>SRPHQWQTDEEGVRTGKCSFPVKYLGHVEVDESRGMHICEDAVKRLKAERKFFKGFFGKTGKKAVKAVLWVSADGLRVVDEKTKDLIVDQTIEKVSFCAPDRNFDRAFSYICRDGTTRRWICHCFMAVKDTGERLSH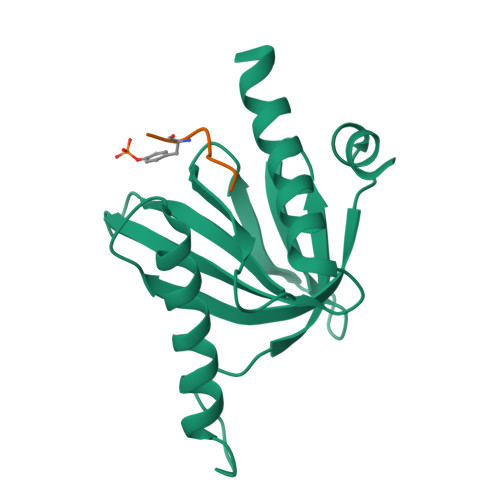AVGCAFAACLERKQKREKE[4x];>[4x]AYIGPYL> STRDYEIQRERIELGRCIGEGQFGDVHQGIYMSPENPALAVAIKTCKNCTSDSVREKFLQEALTMRQFDHPHIVKLIGVITENPVWIIMELCTLGELRSFLQVRKYSLDLASLILYAYQLSTALAYLESKRFVHRDIAA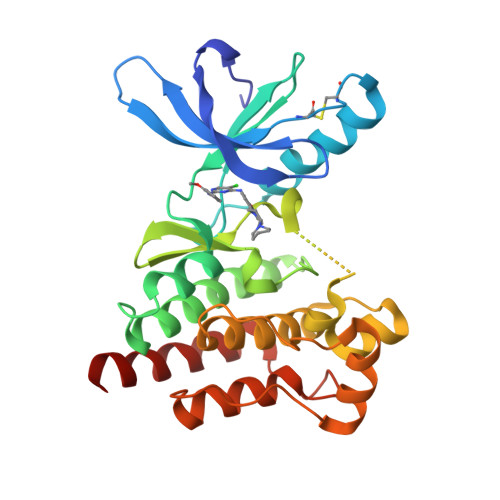RNVLVSSNDCVKLGDFGLSRYMEDSTYYKASKGKLPIKWMAPESINFRRFTSASDVWMFGVCMWEILMHGVKPFQGVKNNDVIGRIENGERLPMPPNCPPTLYSLMTKCWAYDPSRRPRFTELKAQLSTILEEEKLQ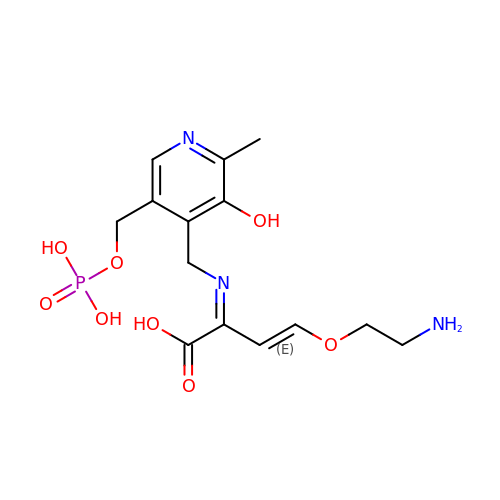(2E,3E)-4-(2-aminoethoxy)-2-[({3-hydroxy-2-methyl-5-[(phosphonooxy)methyl]pyridin-4-yl}methyl)imino]but-3-enoic acid | C14 H20 N3 O8 P | OBCQKAZQAHYUOZ-CALQLVRRSA-N> MRWYPWLRPDFEKLVASYQAGRGHHALLIQALPGMGDDALIYALSRYLLCQQPQGHKSCGHCRGCQLMQAGTHPDYYTLAPEKGKNTLGVDAVREVTEKLNEHARLGGAKVVWVTDAALLTDAAANALLKTLEEPPAETWFFLATREPERLLATLRSRCRLHYLAPPPEQYAVTWLSREVTMSQDALLAALRLSAGSPGAALALFQGDNWQARETLCQALAYSVPSGDWYSLLAALNHEQAPARLHWLATLLMDALKRHHGAAQVTNVDVPGLVAELANHLSPSRLQAILGDVCHIREQLMSVTGINRELLIT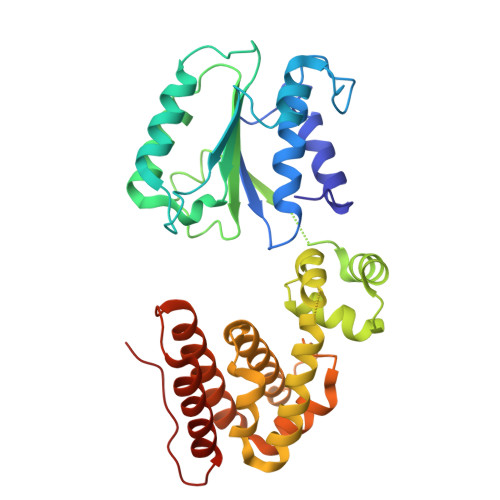DLLLRIEHYLQPGVVLPVPHL>SAAEALREHLGTLEEKMKRHSGLLDIHATQLRTHSEHLQELEATSNDGKLIWKIEDFRNKRESEVKGHPPCLSSVPFHTGPCGYKMASKVY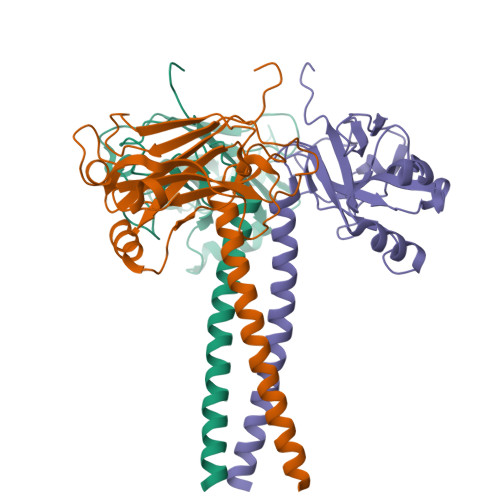LNGDGEGRGTHLSLYVVLMVGDFDALLPWPFRQTVALSVLDQSGAGNHQSLSFKPDLTSKSFQRPTDEKAGNVAVGFSCFIPLIKLEEPQNATYVKEDTMFVKVKVDMVGLEQLLE[2x]The ebolavirus nucleoprotein (NP) is the most abundant protein in infected cells and is essential for viral transcription and replication; thus, it represents an attractive target for therapeutic intervention. Ebolaviruses are filamentous enveloped viruses that contain a negative-sense RNA genome of ∼19 kb. These single-stranded RNAs are covered by multiple copies of nucleoprotein (NP) and are associated with an RNA-dependent RNA polymerase (L), a phosphoprotein polymerase cofactor (VP35), and a transcription activator (VP30). In nonsegmented, negative-sense (NNS) RNA viruses, premature polymerization of the NP and nonspecific binding of cellular RNA is prevented by binding of the newly synthesized NP to the phosphoprotein (P). This interaction builds a complex designated N0-P. Formation of this N0-P complex has been proposed to be key to providing monomeric and RNA-free NPs as a substrate for encapsidation of the viral RNA genome and the formation of the NC.

The capacity of many NNS viruses to prevent premature NP polymerization via the N-terminal domain of the phosphoprotein prompted us to express and purify the chaperone domain of SUDV VP35(1-49) fused to the SUDV NPcore region (residues 34 to 367). Purification of this heterodimer complex allowed us to report the crystal structure of SUDV VP35-NPcore to 2.3-Å resolution. Here, we present the structure of SUDV NP in complex with the amino-terminal portion of the phosphoprotein VP35 at 2.3 Å. This structure captures VP35 chaperoning SUDV NP in a monomeric and RNA-free state. The structure revealed the characteristic bi-lobed configuration expected of the filovirus NP with an RNA-binding cleft in between. The SUDV NPcore contains two major domains, an N-lobe (residues 34 to 340) and a C-lobe (residues 341 to 367), both of which are predominantly α-helical. In this interaction, residues H10 to P12 of VP35 form a beta hairpin (β1), which is stabilized through main-chain hydrogen bonds by a longer beta sheet formed by β4 and β5 of NP. The medial part of VP35, residues S15 to L22, adopts an extended helical conformation (α1) located near the interface defined by the N- and C-lobes of NP. However, the comparison of these structures also revealed two previously unknown interactions between SUDV VP35 and NP: a hydrogen bond (VP35:R5-NP:D275) and a structured beta strand (β1) that complements a beta loop in NP formed by β4 and β5. Importantly, replacement of the amino acid residues involved in the beta strand interaction (VP35:H10G/G11P/P12G) resulted in a dramatic decrease in the dissociation constant (KD of ∼1.34 × 10−5 M). This result suggests that the newly visualized beta sheet interaction is essential for maintaining high-affinity binding between SUDV NP and VP35. NP is maintained in a monomeric and RNA-free state as VP35 occupies this hydrophobic pocket.

> MQQDRTYRHHGPEVSGWFSEQLMTGKIPLTEVFVDVENKPSPAPITIISGIVRQRVIPVYVVNDLEGICQHIIQAFEAGVDFQDNADSFLLLLCLHHAYQGDHRLFLKSDAVQYLEGHGFRFEVREKENVHRLDELLPNVTGGKNLRRTLAAMPEEETTEANAGQFLSFASLFLPKLVVGEKACLEKVQRQIQVHAEQGLIQYPTSWQSVGHMMVIFRLMRTNFLIKFLLIHQGMHMVAGHDANDTVISNSVAQARFSGLLIVKTVLDHILQKTDLGVRLHPLARTAKVKNEVSSFKAALGSLAKHGEYAPFARLLNLSGVNNLEHGLYPQLSAIALGVATAHGSTLAGVNVGEQYQQLREAATEAEKQLQQYAETRELDNLG1-[2-[(1~{R},3~{S},5~{R})-3-[(6-bromanylpyridin-2-yl)carbamoyl]-2-azabicyclo[3.1.0]hexan-2-yl]-2-oxidanylidene-ethyl]indazole-3-carboxamide 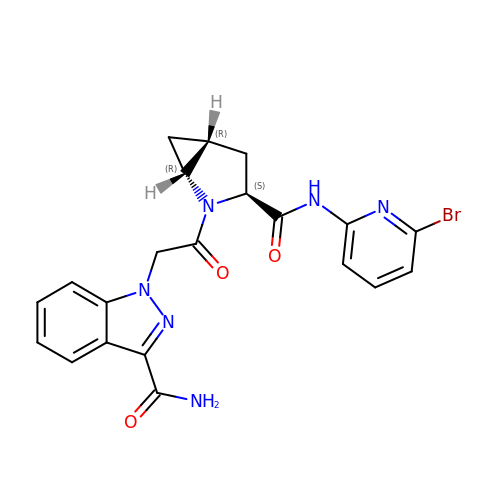| C21 H19 Br N6 O3 | CWZUTHDJLNZLCM-DFBGVHRSSA-N> VEWTDKERSIISDIFSHM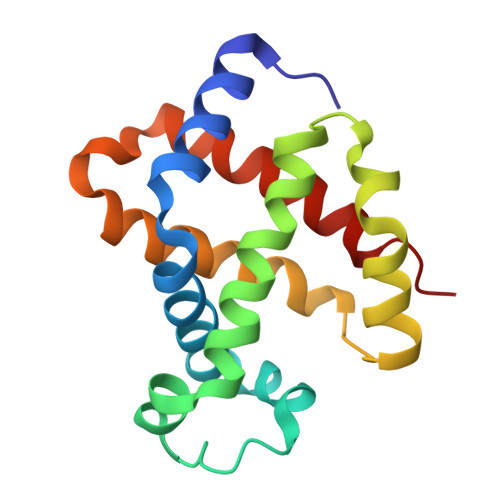DYDDIGPKALSRCLIVYPWTQRHFSGFGNLYNAEAIIGNANVAAHGIKVLHGLDRGVKNMDNIAATYADLSTLHSEKLHVDPDNFKLLSDCITIVLAAKMGHAFTAETQGAFQKFLAVVVSALGKQYH>P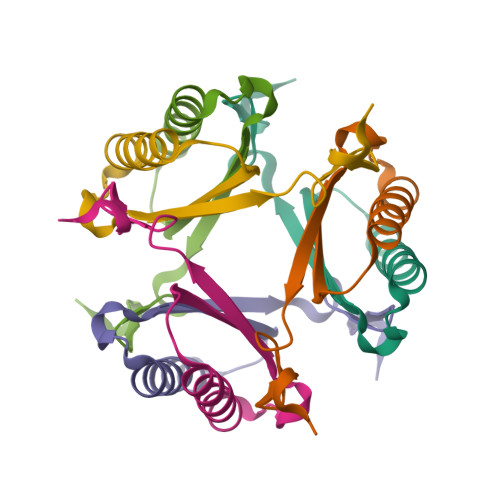YVTVKMLEGRTDEQKRNLVEKVTEAVKETTGASEEKIVVFIEEMRKDHYAVAGKRLSDME[2x]Peptidyl-prolyl isomerases (PPIases) catalyze intrinsically slow and often rate-limiting isomerization of prolyl-peptide bonds in unfolded or partially folded proteins, thereby speeding up the folding process and preventing misfolding. An example of such a protein is SlyD (Sensitive to Lysis D), which consists of an FKBP type PPIase domain and a chaperone domain, called IF (insert-in-flap) domain, that has been shown to exhibit chaperone activity. Each of these domains contains one binding site for unfolded proteins or peptides. Often, FKBPs are linked to an additional chaperone domain that can increase their PPIase activity by up to 200-fold.

Although most of the protein–peptide complexes did not crystallize or yielded crystals of poor diffraction quality, we succeeded in structure determination for four complexes of SlyDWT with bound substrates: psWT, W4A, W4K, and M8A. In all structures, the peptide substrates are bound in the PPIase binding pocket with the proline residue in cis conformation, coordinated by the previously observed protein–peptide polar interactions, namely N35-L9, I37-L9, Y63-F11, H119-F11 and Y92-F13. Although all peptide substrates bound to both SlyDWT domains in solution, the chaperone domains displayed no electron density for peptide substrates psWT and M8A in their respective crystal structures. The absence of these substrates in the high-affinity chaperone domains can be attributed to high dynamics of substrate binding and serendipitous blocking of the binding site by neighbouring molecule of SlyD in the crystal packing. An interesting exception to the coupling of the substrate affinity and protein activity is the mutation M8A that slightly reduces the peptide binding affinity but significantly increases the protein activity. The mutation of methionine 8 to alanine removes the hydrophobic interactions mediated by the methionine side chain, as is visible in the crystal structure and thus facilitates proline isomerization. Thus, the M8 side chain of the peptide substrate has an influence on the enzymatic activity of SlyD, which is not caused by a change in the overall binding mode of the peptide. Finally, the loose conformation is defined by the newly determined structures with the substrate bound only in the FKBP domain. In these structures, the access to the FKBP binding site is not restricted and the peptides bound in the FKBP domain can freely diffuse from the binding site upon its release.

> MKVGQDKVVTIRYTLQVEGEVLDQGELSYLHGHRNLIPGLEEALEGREEGEAFQAHVPAEKAYGPHDPEGVQVVPLSAFPEDAEVVPGAQFYAQDMEGNPMPLTVVAVEGEEVTVDFNHPLAGKDLDFQVEVVKVREATPEELLHGHAHPSGHHHHHH;> TRYWNAKALPFAFGA>MAKVFSRCELAKEMHDFGLDGYRGYNLADWVCLAYYTSGFNTNAVDHEADGSTNNGIFQISSRRWCRTLASNGPNLCRIYCTDLLNNDLKDSIVCAMKIVQEPLGLGYWEAWRHHCQGRDLSDWVDGCDFLE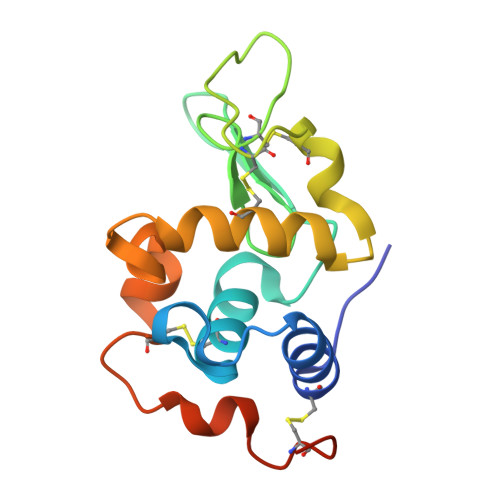HHHHHH[3x]N-[2-({[5-(DIMETHYLAMINO)NAPHTHALEN-1-YL]SULFONYL}AMINO)ETHYL]-2-IODOACETAMIDE 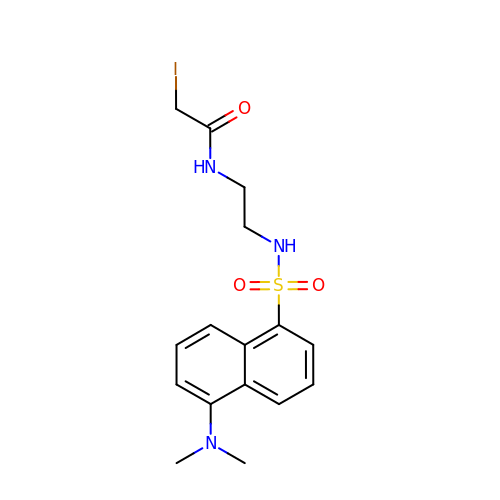| C16 H20 I N3 O3 S | QDHGMMDEGVINBU-UHFFFAOYSA-N> STVVMADVSQYHVNHLVTFCLGEEDGVHTVEDASRKLAVMDSQGRVWAQEMLLRVSPSQVTLLDPVSKEEL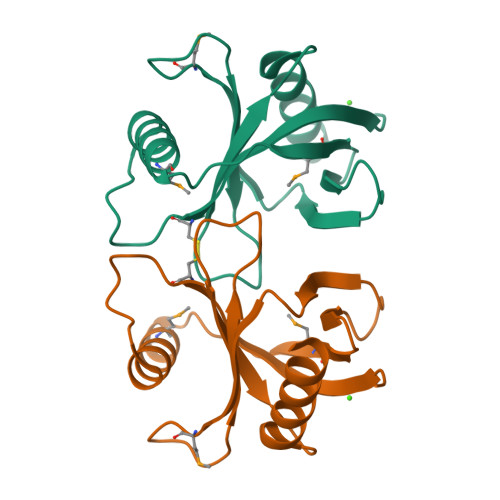ESYPLDAIVRCDAVMPRGRSRSLLLLVCQEPERAQPDVHFFQGLLLGAELIREDIQGALQNYRSGRGER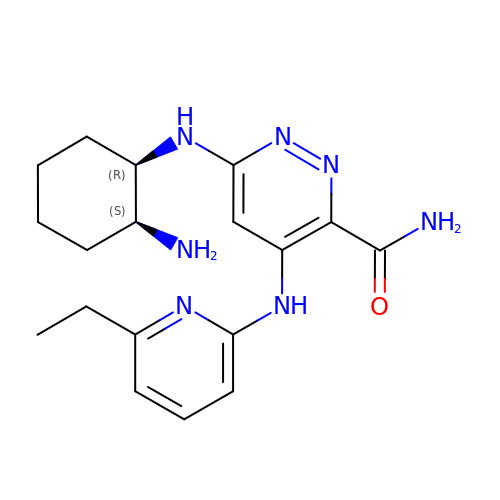6-{[(1R,2S)-2-aminocyclohexyl]amino}-4-[(6-ethylpyridin-2-yl)amino]pyridazine-3-carboxamide | C18 H25 N7 O | WDVJRXQKCPLXTN-QWHCGFSZSA-N>GPLGSMEKNMRPYTVLWADDEIDLLKPHILFLEQKGYQVTPVLSGNDAIEAVQNNDFDIVFLDENMPGIGGLDALQKIKELKPYTPVVMITKSEEEHIMTQAIGGKIADYLIKPVNPNQLLLSLKKNLQQHSIISETTNTNYRQEFVQLGTQMSGKLSFEEWKELYRRIVFWEIELEQADRQMGELLEMQKQEANRLFARFVTQNYREWIAKPDTRPTMSPDLFKQKVFPLLDNGEKVFFILIDNFRQDQWESVKSMLSEFYTFEEDMYLSILPTATQYARNAIFSGLMPLQIEKMFPDLWVDEESEEGKNLNEEPMIRTLIERYRKHYSFSYNKVYETKFGERLLGQIRSLSQNQLNVIVLNFVDMMSHARTDSKMIRELASNEAAYRSLTKSWFKHSTTYNLFRSIAEMGY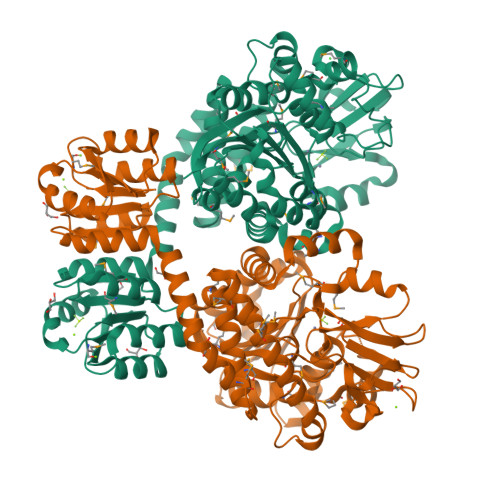KVVLTTDHGTIQVKNPVKVIGDRSTNTNLRYKIGKNLDYNPKEVFEIKDPASVGLPHNNLSDKFIFTKEDDFFAYPNNYNYYVQYYRNTFQHGGISLEEMLVPVITMQPK[4x]>MAKKTSSAPRTVLPFEAMPQHPGNRWLRLLQIWREQGYEHLHLEMHQTFQELGPIFRYNLGGPRMVCVMLPEDVEKLQQVDSLHPCRMILEPWVAYRQHRGHKCGVFLLNGPEWRFNRLRLNPDVLSPKAVQRFLPMVDAVARDFSQALKKKVLQNARGSLTLDVQPSIFHYTIEASNLALFGERLGLVGHSPSSASLNFLHALEVMFKSTVQLMFMPRSLSRWISPKVWKEHFEAWDCIFQYGDNCIQKIYQELAFNRPQHYTGIVAELLLKAELSLEAIKANSMELTAGSVDTTAFP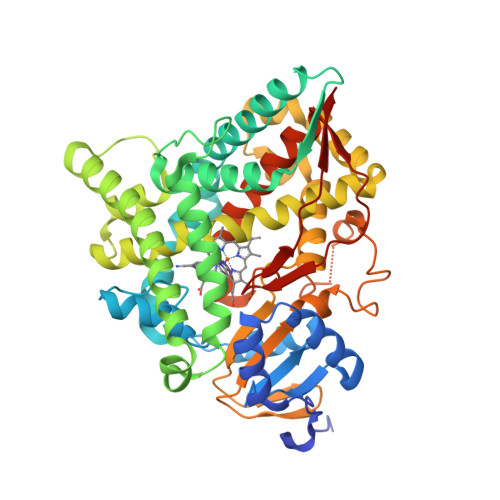LLMTLFELARNPDVQQILRQESLAAAASISEHPQKATTELPLLRAALKETLRLYPVGLFLERVVSSDLVLQNYHIPAGTLVQVFLYSLGRNAALFPRPERYNPQRWLDIRGSGRNFHHVPFGFGMRQCLGRRLAEAEMLLLLHHVLKHFLVETLTQEDIKMVYSFILRPGTSPLLTFRAINHHHH[12x]trichloromethane 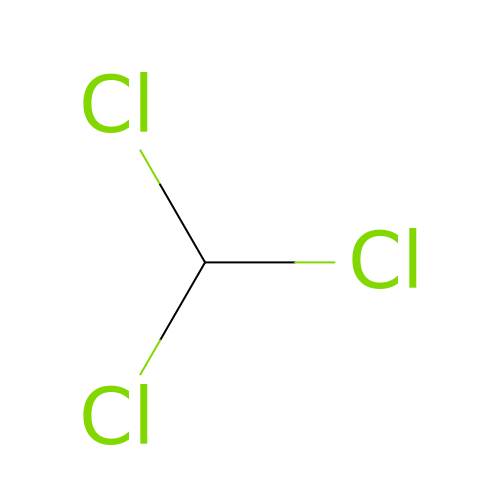| C H Cl3 | HEDRZPFGACZZDS-UHFFFAOYSA-N> MLEESAVTRGKWMLAAAWAVVLVGARVHGAELNTLRGLDVSRTGSGAQVVVTGTRPPTFTVFRLSGPERLVVDLSSADATGIKGHHEGSGPVSGVVASQFSDQRASVGRVLLALDKASQYDVRADGNRVVISVDGTSQSVDAKRAETPARTERMTASVEAKPHPVAAQAPAKVVKAESAAVPKAALPENVVAAEADEREVSNPAQHITAMSFADDTLSIRADGDIARYEVLELADPPRLAVDLFGVGLATRAPRVKSGALRDVRVGAHADKVRLVLDVRGTMPAYRVDRANRGLEVVLGRAVARTWRRPLRPRAVVASVAEVEPLRQTPVKSDASPVVEVKDVRFEESSSGGRIVMKLSG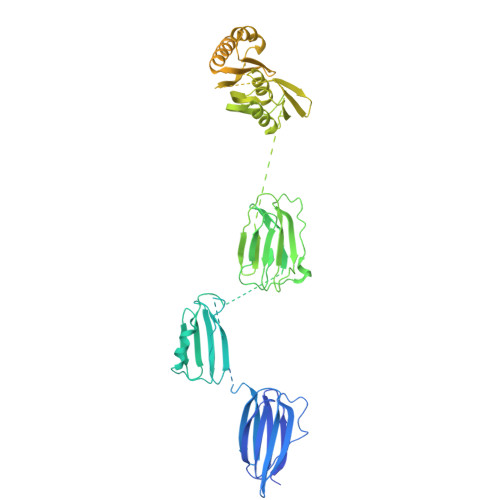TSGWKVDRPDPRSAVLTLDNARLPKKFERSLDTSALDTPVKMISAFSVPGAGGKVRLVVAADGAIEEKVSQSAGTLSWRLDVKGVKTEEVAVAQRTAGFTTEAPAYAAEGAPQQARYRGKRVSFEFKDIDIQNLLRVIAEISKKNIVVADDVSGKVTIRLRNVPWDQALDLVLRTKALGKEEFGNIIRIAPLKTLEEEARLRQERKKSLQQQEDLMVNLLPVNYAVAADMAARVKDVLSERGSVTVDQRTNVLIVKDVRSNTERARSLVRSLDTQTPQVLIESRIVEANTSFSRSLGVQWGGQARAGQATGNSTGLIFPNNLAVTGGVTGTGAGLPDNPNFAVNLPTGTGQGVGGAMGFTFGSAGGALQLNLRLSAAENEGSVKTISAPKVTTLDNNTARINQGVSIPFSQTSAQGVNTTFVEARLSLEVTPHITQDGSVLMSINASNNQPDPSSTGANGQPSIQRKEANTQVLVKDGDTTVIGGIYVRRGATQVNSVPFLSRIPVLGLLFKNNSETDTRQELLIFITPRILNRQTIAQTL> MQPRRMAGHFNPTPQANSLAATHYAHTPELRHMADGAAMSLSGQRIPLLKPTLSKWSRQLRSDIYDELLKLPLRYALHDFRTLQAHIHAVPATATNASCTAAAGERLPPGVYHASSGLSSASPDAPAYYAVAGRDSAVGYAPPLGPADPVDVIPFFVHRSSNGHLPGKVYSMNAKTLMPAFYMRIQNIEGDMFR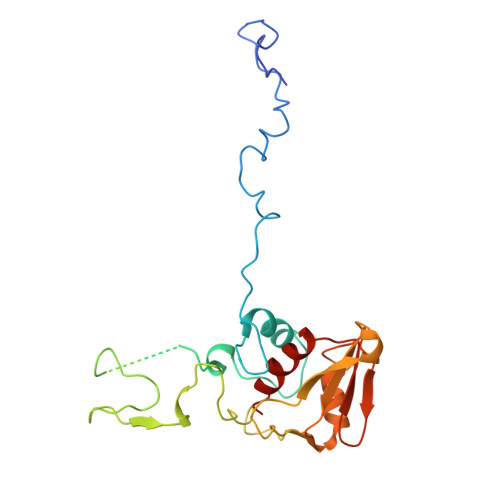FEEELMKIFPTKKIFVRSHSVYVYNVNLDGRAVLHHWLLGLGF> MAYQGFTKLG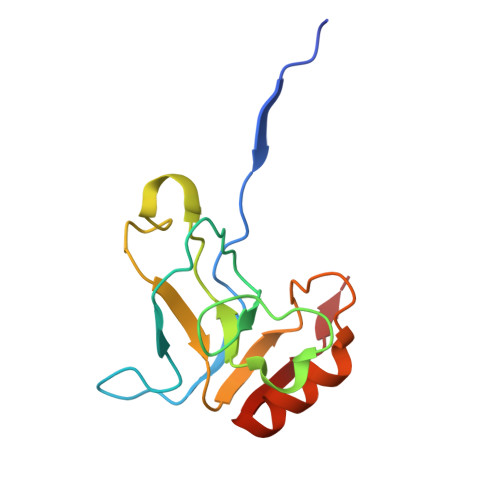EREPLNDIILWEEITPTGHSRKEYAPVASTEYRVGEVLKADGSKVAAGQEAQADSVCIVNFYADLQLSYHGQLKVVGIYRDAELKDLLKLESGVDAAAVKSALKAKGIDFVPTGL>MDPEQIKTALGSGLLSFPVTHFDAEGRFAADSYREHVEWLAGYKAPVLFAAGGTGEFFSLKPDEIPTIVAAAKEVAGE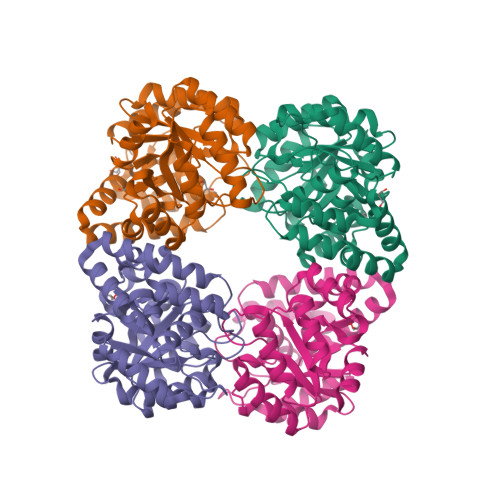TAIVSGCGYGTEIAVDIARSVEKVGADGILLLPHYLIDAPQEGLYAHIKKVCQSVGIGVMVYNRDNSVLQADTLARLCDECPNLVGFKDGTGDIGLVRQITAKMGDRLMYLGGMPTAELFAEAYLGAGFTTYSSAVFNFVPGLANEFYAALRAGERATCERILVDFFYPFMAIRNRAKGYAVSAVKAGVRLQGFNAGPVRAPLKDLTNEEIGMLEALIGTHKRKAWSHPQFEK[4x]> AAAAAAMTMMDMNF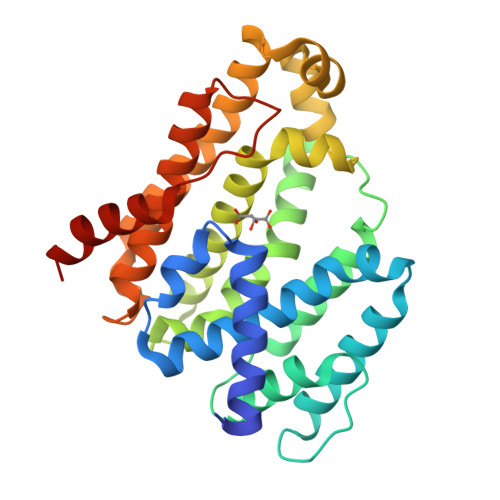KYCHKIMKKHSKSFSYAFDLLPEDQRKAVWAIYAVCRKIDDSIDVYGDIQFLNQIKEDIQSIEKYPYEYHHFQSDRRIMMALQHVAQHKNIAFQSFYNLIDTVYKDQHFTMFETDAELFGYCYGVAGTVGEVLTPILSDHETHQTYDVARRLGESLQLINILRDVGEDFENERIYFSKQRLKQYEVDIAEVYQNGVNNHYIDLWEYYAAIAEKDFRDVMDQIKVFSIEAQPIIELAARIAIEILDEVRQANYTLHERVFVEKRKKAKLFHEINSKYHRI>[12x]MRVQFPTT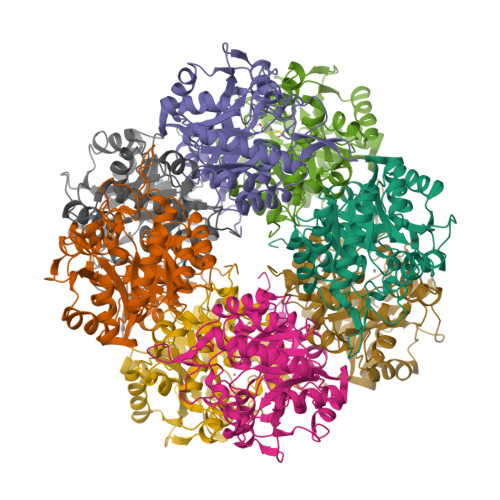RPRRLRASKIIRDAVAETQIDAGDFIYPLFVKPGGEREPIGPMPGIYRWPVGRELINHVEEALSLGINKFILFGVLPDELKNPEGTGGYDPEGVVPRAIRLIKEIFGDRVLVFADVCLCEYTDHGHCGVVKEKRDRWYVDNDETIKLYAKEAVVYAEAGADFVAPSGMMDGQVREIRRALDAHGFEEVGIMAYSAKYASAFYGPFRVAAASAPKFGDRRTYQMDPRNAYEALKEVAMDLEEGADIVMVKPALAYLDVIRLVKQHFPWVPLAAYNVSGEYSLVKAAATAGYVDERTITLEILTAIKRAGADLILTYHALEAAKWIKEGLPF> MRNQELARIFEEIGLMSEFLGDNPFRVRAYHQAARTLYDLDTPIEEIAEKGKEALMELPGVGPDLAEKILEFLRTGKVRKHEELSRKVPRGVLEVMEVPGVGPKTARLLYEGLGIDSLEKLKAALDRGDLTRLKGFGPKRAERIREGLALAQAAGKRRPLGAVLSLARSLLEAIRALPGVERAELCGSARRYKDTVGDLDFLVASREGERAVEGFVRLPQVKEVYAKGKERATVFLKNGLQVDLRVVPPESYGAGLQYLTGSDAHSIRLRALAQEKGLKLSE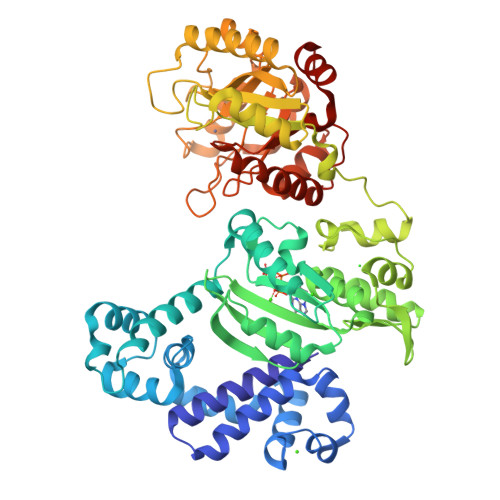YGVFRGEKRIAGETEEEVYAALGLPWIPPPLREDQGEVEAALEGRLPKLLELPQVKGDLQVHSTYSDGQNTLEELWEAAKTMGYRYLAVTDHSPAVRVAGGPSPEEALKRVGEIRRFNETHGPPYLLAGAEVDIHPDGTLDYPDWVLRELDLVLVSVHSRFNLPKADQTKRLLKALENPFVHVLAHPTARLLGRRAPIEADWEAVFQKAKEKGVAVEIDGYYDRMDLPDDLARMAYGMGLWISLSTDAHQTDHLRFMELAVGTAQRAWIGPERVLNTLDYEDLLSWLKARRGV pyrazolo[5,1-a]phthalazin-6-amine | C10 H8 N4 | 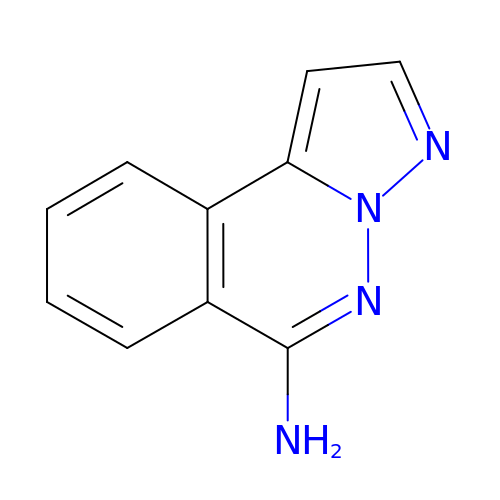VOLKDTKFDOIYJN-UHFFFAOYSA-N ADENOSINE-5'-PHOSPHATE-2',3'-CYCLIC PHOSPHATE | C10 H13 N5 O9 P2 | 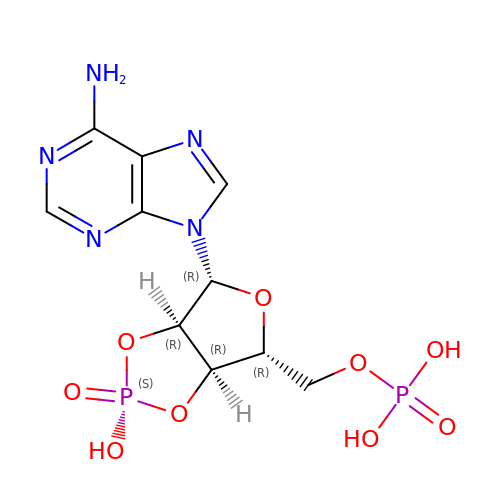HJMBCNJTGVMDOA-KQYNXXCUSA-N> MGTALLQRGGCFLLCLSLLLLGCWAELGTGATFPKAMDNVTVRQGESATLRCTIDNRVTRVAWLNRSTILYAGNDKWCLDPRVVLLSNTQTQYSIEIQNVDVYDEGPYTCSVQTDNHPKTSRVHLIVQVSPKIVEISSDISINEGNNISLTCIATGRPEPTVTWRHISPKAVGFVSEDEYLEIQGITREQSGDYECSASNDVAAPVVRRVKVTVNYPPYISEAKGT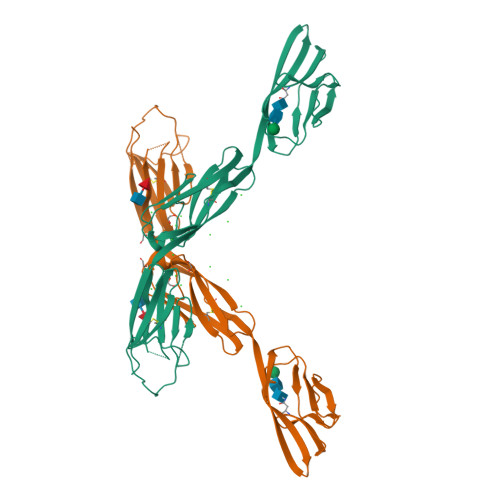GVPVGQKGTLQCEASAVPSAEFQWYKDDKRLIEGKKGVKVENRPFLSKLIFFNVSEHDYGNYTCVASNKLGHTNASIMLFTSHHHHHH>MDTLFDAPGRSQFVPADQAFAFDFQQNQHDLNLTWQIKDGYYLYRKQIRITPEHAKIADVQLPQGVWAGGSEIY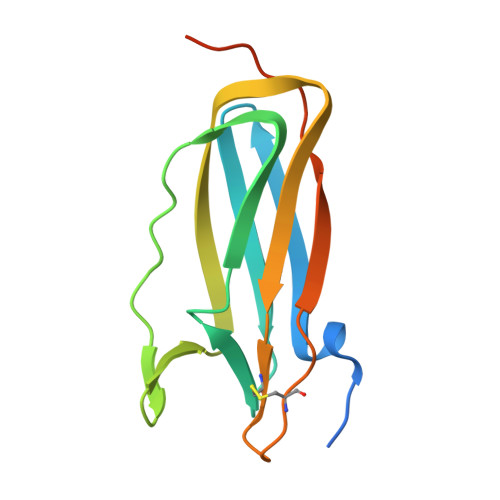RDRLTLPVTINQASAGATLTVTYQGCADAGFCYPPETKTVPLSEVVANNAAPQPVGLVPR[2x]The sliding clamp PCNA (proliferating cell nuclear antigen) is a central player in multiple aspects of chromosomal DNA replication, repair and genome stability. This ring-shaped homotrimer encircles double-stranded DNA to act as a processivity factor for DNA polymerases and a landing pad for the assembly of various DNA processing factors such DNA ligase I, the flap endonuclease Fen1, and the clamp loader complex replication factor C (RF-C) which opens and closes the PCNA ring around dsDNA. Many of the proteins that interact with PCNA, including DNA polymerase δ, DNA ligase I, Fen1 and RF-C, do so via a common mechanism that involves a short linear interaction motif on the partner protein called a PCNA-interacting protein (PIP) motif. The best characterised PIP motifs have conserved sequence Qxxψxxθθ, where ψ and θ represent amino acids with hydrophobic and aromatic side chains, respectively, but other variations on this sequence (so-called non-canonical PIP motifs) have been identified such as ψxxxθ and Qxxψxθ.

The p50 (PolD2, Pol31) and p66 (PolD3, Pol32) subunits of Pol δ are also found as components of the trans-lesion synthesis DNA polymerase Pol ζ, in complex with the Pol ζ catalytic subunit REV3L (yeast Rev3) and two copies of the accessory subunit REV7 (Rev7). The conserved PIP motif found at the extreme C-terminus of human, S. cerevisiae and S. pombe PolD3 orthologues is readily identifiable at the C-terminal end of the Ct PolD3 protein (sequence: 441 QGSIMSWF 448 conserved PIP motif residues underlined). The Ct PolD3 peptide (sequence: 437GKGGQGSIMSWFAKK451 with conserved PIP motif residues underlined) occupied a single PIP binding site only, with the other sites on Ct PCNA being occluded by crystal packing (specifically, by the loop that spans residues Thr186-Lys190 in neighbouring symmetry mates). Only 11 of 15 residues in the peptide could be seen in the electron density map (Gln441 to Lys451) suggesting that the N-terminal four residues of the peptide are flexible. Consistent with the high degree of conservation of the PIP peptide sequence at the C-terminal end of PolD3 orthologues, the mode of PCNA-PIP binding observed is strictly canonical: part of the peptide adopts a 310 helical structure, Ct PolD3 Gln441 inserts into the Q-pocket on Ct PCNA and Ct PolD3 Ile444 and Phe448 form a 2-fork plug that inserts into the hydrophobic surface pocket on Ct PCNA. Ct PolD3 Gln441(OE1) makes water-mediated hydrogen bonding interactions with Ser208 (N) and Ala252 (O) on Ct PCNA, Gly442 (N) hydrogen bonds with Pro253 (O), Ser 443 (OG) and Ile444 (N) both hydrogen bond with His44(O), Trp447 (NE1) hydrogen bonds with Glu232 (O), Ala449 (O) with Gly127 (N), and Lys451 (N) with His125 (O). Hydrophobic interactions with Ct PCNA are seen with Ct PolD3 Gln441, Gly442, Ile444, Met445, Trp447 and Phe448.

>[3x]GAMALEARLEQASILKKVVDAIKDLVQDCNFDCNDSGIALQAMDNSHVALVSMMLKAEGFSPYRCDRNIALGVNLTSLTKVLRAAQNEDILTLKAEDAPDVLNLVFESSETDRISEYDLKLMDIDQEHLGIPETEYAATITMPSNEFKRITTDLMAMSESVTIEANKDGVKFSCQGDIGNGSVTLRQHTNVEKPNESIEIELSEPVSLTFSLKYLVNFCKASALSNTVKICLSNEVPLLVEYSLGGSSYLRFYLAPKIGDDE;> GKGGQGSIMSWFAKK>VGPKTGEENQVLVPNLNPTPENLEVVGDGFKITSSINLVGEEEADENAVNALREFLTANNIEINSENDPNSTTLIIGEVDDDIPELDEALNGTTAENLKEEGYALVSNDGKIAIEGKDGDGTFYGVQTFKQLVKESNIPEVNITDYPTVSARGIVEGFYGTPWTHQDRLDQIKFYGENKLNTYIYAPKDDPYHREKWREPYPESEMQRMQELINASAENKVDFVFGISPGIDIRFDGDAGEEDFNHLITKAESLYDMG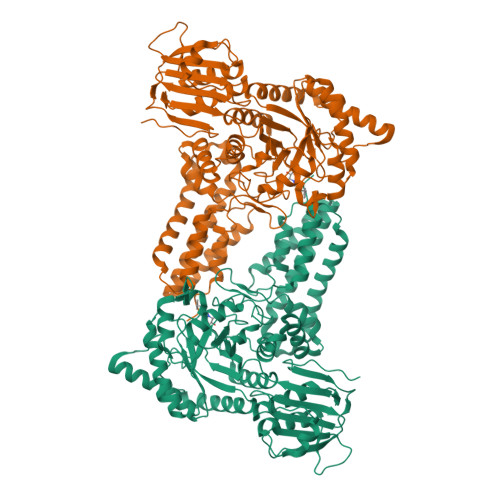VRSFAIYWDDIQDKSAAKHAQVLNRFNEEFVKAKGDVKPLITCPTEYDTGAMVSNGQPRAYTRIFAETVDPSIEVMWTGPGVVTNEIPLSDAQLISGIYDRNMAVWWNYPVTDYFKGKLALGPMHGLDKGLNQYVDFFTVNPMEHAELSKISIHTAADYSWNMDNYDYDKAWNRAIDMLYGDLAEDMKVFANHSTRMDNKTWAKSGREDAPELRAKMDELWNKLSSKEDASALIEELYGEFARMEEACNNLKANLPEVALEECSRQLDELITLAQGDKASLDMIVAQLNEDTEAYESAKEIAQNKLNTALSSFAVISEKVAQSFIQEALSFDLTLI[2x]>[4x]RSELRFDPGTSNRNFRIAASDFGQALML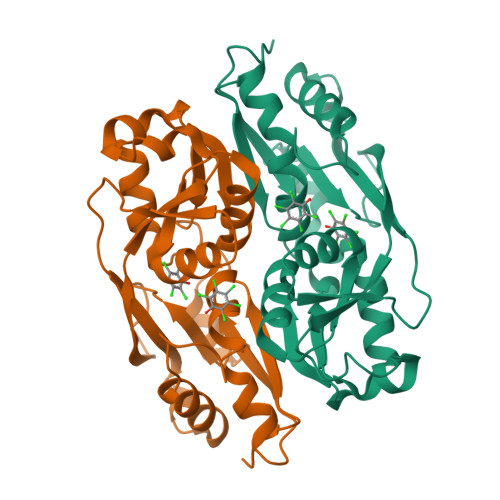PRLYATLEETAPQVRVTGVNLRHGPLVEELESGSIDIAFGGFPTLSAGIKTQTLFREEYVCVMRQSHPALTHGLDLEAFRQCRHIIVTAHEFNHVHEQVEARLLELLPPESIRFTTENFLVSAVIAEETDVILTIPSRLARWFANRGGLTIFPVPIELPSIEVKQYWHERYDKDPGNIWLRRVIAKIGFQNPPAE>[2x]MGSSVLASCPKKPVSSYLRFSKEQLPIFKAQNPDAKTTELIRRIAQRWRELPDSKKKIYQDAYRAEWQVYKEEISRFKEQ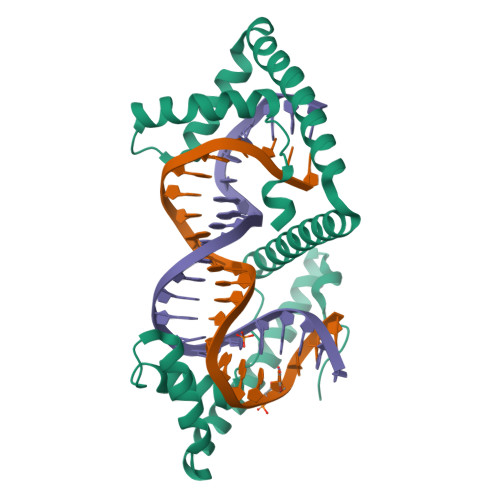LTPSQIMSLEKEIMDKHLKRKAMTKKKELTLLGKPKRPRSAYNVYVAERFQEAKGDSPQEKLKTVKENWKNLSDSEKELYIQHAKEDETRYHNEMKSWEEQMIEVGRKDLLRRTIKKQRKYGAEECLQHHHHHH7-aminoheptanoic acid | C7 H15 N O2 | 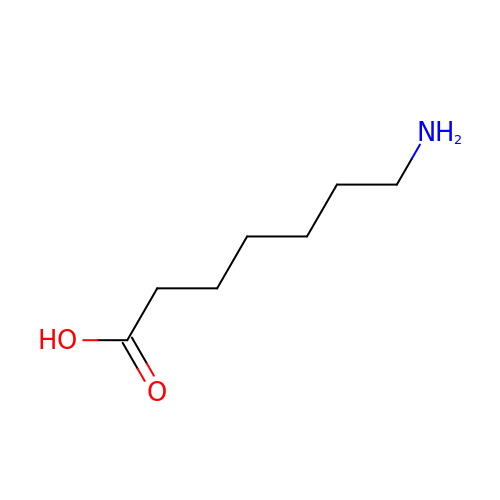XDOLZJYETYVRKV-UHFFFAOYSA-N>[4x]MRIVPFGAAREVTGSAHLLLAGGRRVLLDCGMFQGKEEARNHAPFGFDPKEVDAVLLTHAHLDHVGRLPKLFREGYRGPVYATRATVLLMEIVLEDALKVMDEPFFGPEDVEEALGHLRPLEYGEWLRLGALSLAFGQAGHLPGSAFVVAQGEGRTLVYSGDLGNREKDVLPDPSLPPLADLVLAEGTYGD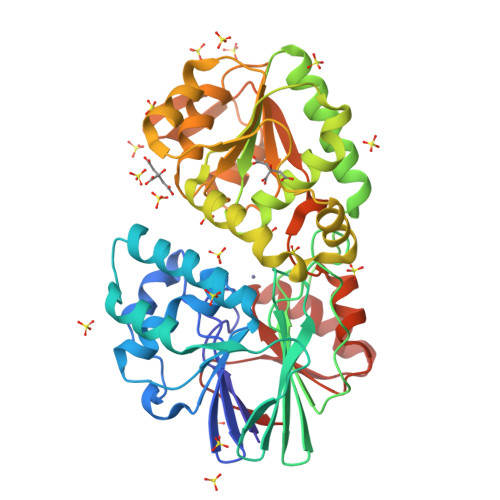RPHRPYRETVREFLEILEKTLSQGGKVLIPTFAVERAQEILYVLYTHGHRLPRAPIYLDSPMAGRVLSLYPRLVRYFSEEVQAHFLQGKNPFRPAGLEVVEHTEASKALNRAPGPMVVLAGSGMLAGGRILHHLKHGLSDPRNALVFVGYQPQGGLGAEIIARPPAVRILGEEVPLRASVHTLGGFYGHAGQDELLDWLQGEPRVVLVHGEEEKLLALGKLLALRGQEVSLARFGEGVPV We also show that the purified proteins encoded by PA1502 and PA1500 have glyoxylate carboligase (Gcl) and tartronate semialdehyde (TSA) reductase (GlxR) activity, respectively, in vitro. Gcl condenses two molecules of glyoxylate to yield TSA, which is then reduced by GlxR to yield d-glycerate. GlxR displayed much greater specificity (kcat/KM) for Gcl-derived TSA than it did for the TSA tautomer, hydroxypyruvate. P. aeruginosa GlxR was a tetramer in solution, whereas Hyi formed a dimer.

GlxR was crystallized from drops containing 0.1 M sodium acetate (pH 4.5) and 25% (w/v) polyethylene glycol smear medium and from drops containing 0.1 M Tris-HCl (pH 8.5), 20% (w/v) polyethylene glycol smear high and 20% glycerol. The resulting X-ray structures were designated the α and β forms, respectively. The structure of the α form was solved to 2.07 Å resolution and the structure of the β form was solved to 2.21 Å resolution. Both conformers contain an N-terminal domain comprised of nine α-helices surrounding a core of nine β-strands, and an exclusively α-helical C-terminal domain. By contrast, the oligomeric arrangement of the β form tetramer adopts a more open, expanded structure. However, when we superimposed the individual α and β protomers, they had a very similar structure, indicating that the differences in quaternary structure are primarily due to rigid body rearrangements of the protomers. Given that inter-protomer contacts in both the α and β forms of the enzyme are mediated through interactions between the C-terminal domains, this rigid body movement can be thought of as a rocking motion around a C-terminal pivot point. Interestingly, and although the α conformer is more ‘compact’ than the β conformer, the distance between the serine –OH and the lysine –NH3+ was larger in GlxRα (5.3 Å) than it was in GlxRβ (4.6 Å). Given that the GlxRβ tetramer is also structurally more similar (cf. the GlxRα tetramer) to the GarRSty tetramer, these data suggest that the GlxRβ conformer is likely to be more physiologically relevant. By contrast, the GlxRβ conformer – at both the protomer and tetramer level of organization – was a better fit than GlxRα with the X-ray crystal structure of a GlxR homologue, GarRSty.

>MGHHHHHHAENLYFQHMAKIGFIGTGIMGKPMAQNLQKAGHSLFLSTHHDAAPADLLEAGAIALANPKEVAQEAEFIIVMVPDTPQVEDVLFRKDGIAEGAGPNKVVIDMSSISPTATKGFAEKIKATGAQYLDAPVSGGEVGAKAATLSIMVGGCPNTFERALPLFQAMGKNITRVGGNGDGQTAKVANQIIVALNIQAVAEALLFAARNGADPAKVREALMGGFASSRILEVHGERMVKGTFDPGFRISLHQKDLNLALAGARELNLNLPNTANAQQVFSTCAAIGGSNWDHSALIKGLEHMANFSIRDE[4x]> GPGSEFGHSDAQTLAMMLQEQLDAIN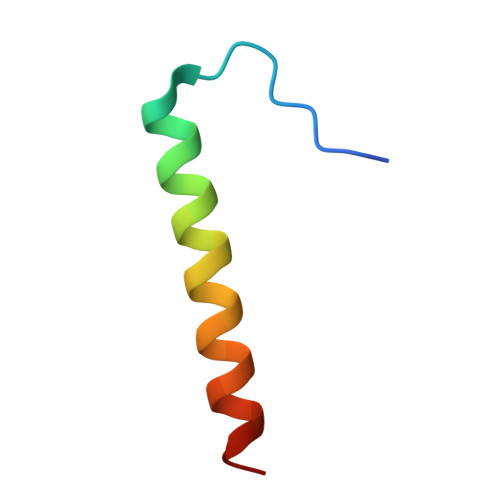KEIRLIQEEK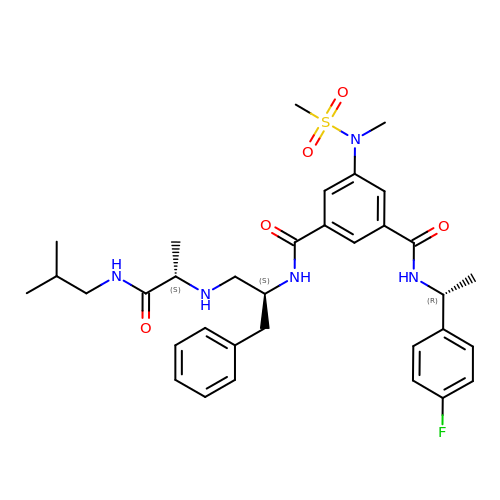N-[(1S)-1-benzyl-2-{[(1S)-2-(isobutylamino)-1-methyl-2-oxoethyl]amino}ethyl]-N'-[(1R)-1-(4-fluorophenyl)ethyl]-5-[methyl(methylsulfonyl)amino]isophthalamide | C34 H44 F N5 O5 S | FZTXBRKPIRTQCY-QEGDFHJFSA-N> GPGSEVPADGNAGLLAEPQIAMFCGKLNMHMNVQNGKWESDPSGTKTCIDTKEGILQYCQEVYPELQITNVVEANQPV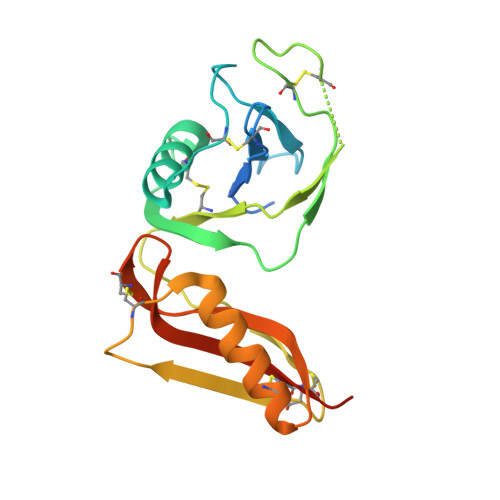TIQNWCKRGWKQCNGHPHIVVPYRCLVGEFVSDALLVPDKCKLLHQERMDVCETHLHWHTVAKESCSEKSMNLHDYGMLLPCGIDKFRGVEFVCCPLAEESDNLDS>MDSGRLAVIALGGNAIAGPGMDVSVESQTAAVKRASSIIADVLADGWRSVITHGNGPQVGYLSEAFEALPPERPRQPLYIATAMTQAWIGLLLKHSLEEELRRRGLNVLVPVVISRVLVDVSDPSFNNPSKPVGPIYGREEAEELSRRYGWVFKRDPRGGFRRVVPSPRPVSIVDRDLIAEASAESPAVVALGGGGVPV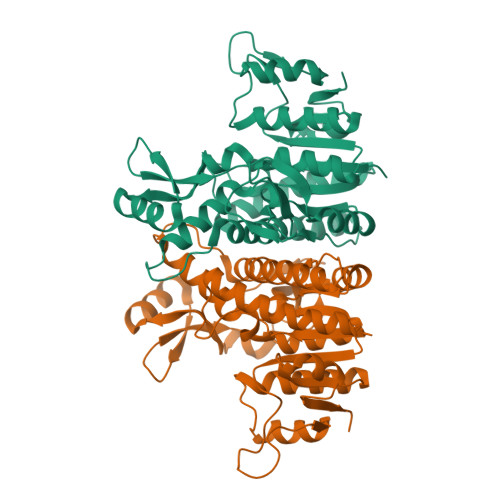VERPGGVLEPVEAVVDKDLASSLLATQLNADLLVILTDVPGVAVNYGREGERWLRRAAASELKKYLREGHFPPGSMGPKVEAAISFVERTGKPAVIGSLEEARQVLSLQAGTVVMLG[2x]> GSAAASPAWMPAYACQRPTPLTHHNTGLSEALEILAEAAGFEGSEGRLLTFCRAASVLKALPSPVTTLSQLQGLPHFGEHSSRVVQELLEHGVCEEVERVRRSERYQTMKLFTQIFGVGVKTADRWYREGLRTLDDLREQPQKLTQQQKAGLQHHQDLSTPVLRSDVDALQQVVEEAVGQALPGATVTLTGGFRRGKLQGHDVDFLITHPKEGQEAGLLPRVMCRLQDQGLILYHQHQHSCCESPTRLAQQSHMDAFERSFCIFRLPQPGSWKAVRVDLVVAPVSQFPFALLSWTGSKLFQRELRRFSRKEKGLWLN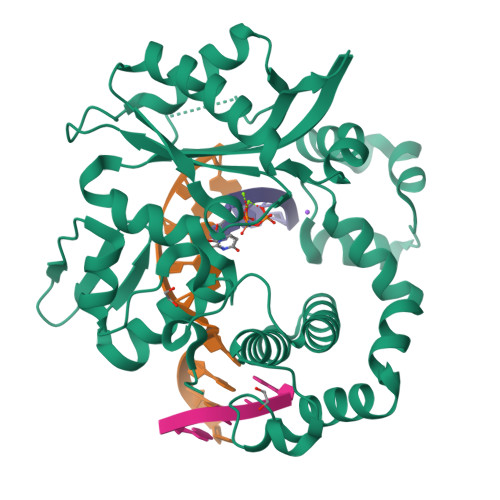SHGLFDPEQKTFFQAASEEDIFRHLGLEYLPPEQRNA> SHMEQLKCCSGILKEMFAKKHAAYAWPFYKPVDVEALGLHDYCDIIKHPMDMSTIKSKLEAREYRDAQEFGADVRLMFSNCYKYNPPDHEVVAM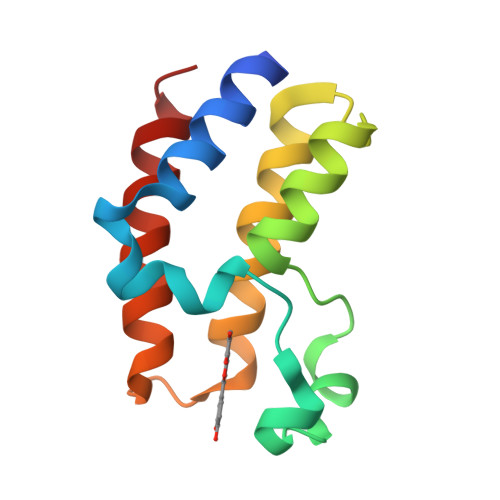ARKLQDVFEMRFAKM>[2x]MIRVYIALGSNLAMPLQQVSAAREALAHLPR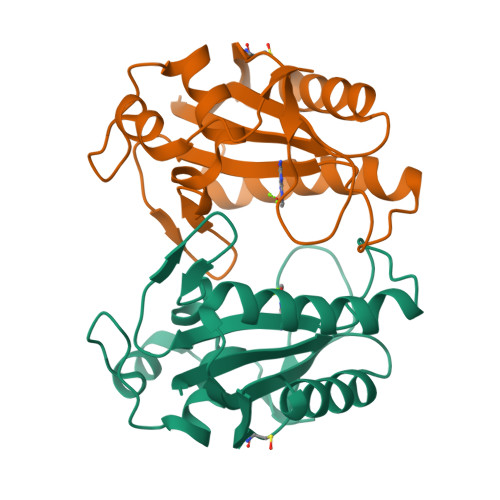SRLVACSPLYRTKPLGPQDQPDFLNAVVALDTSLPPEQLLDHTQAIERNQGRVRKEQRWGPRTLDLDIMLYGDQVIKTDRLTIPHYGLKAREFMLYPLADIAPDLIFPDGESLSECLKRVDKNGLVLW> KITPNLAEFAFSL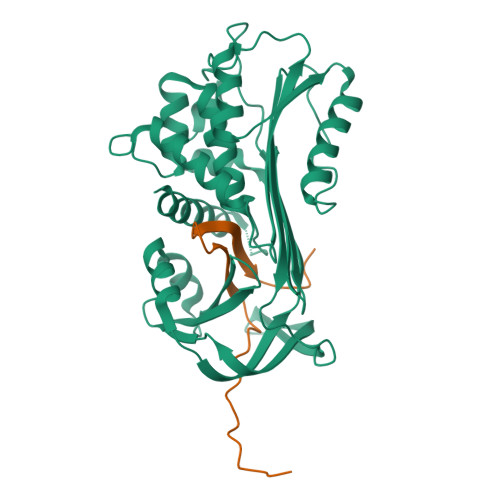YRQLAHQSSTNIFFSPVSIATAFAMLSLGTKADTHDEILEGLNFNLTEIPEAAIHEGFQELLRTLNQPDSQLQLTTGNGLFLSEGLKLVDKFLEDVKKLYHSEAFTVNFGDTEEAKKQINDYVEKGTQGKIVDLVKELDRDTVFALVNYIFFKGKWERPFEVKDTEEEDFHVDQVTTVKVPMMKRLGMFNIQHCKKLSSWVLLMKYLGNATAIFFLPDEGKLQHLENELTHDIITKFLENDRRSASLHLPKLSITGTYDLKSVLGQLGITKVFSNGADLSGVTEEAPLKLSKAVHKAVLTIDEKGTEAAGAMF;> LEAIPRSIPPEVKFNAPFVFLMIEQNTKSPLFMGKVVNPTQK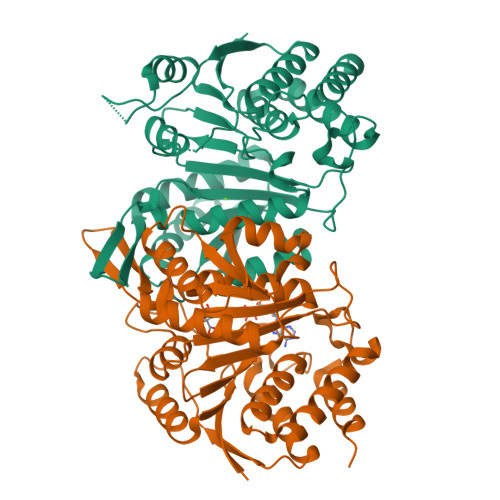> MGSTGGVQTVTLIPGDGIGPEISAAVMKIFDAAKAPIQWEERNVTAIQGPGGKWMIPSEAKESMDKNKMGLKGPLKTPIAAGHPSMNLLLRKTFDLYANVRPCVSIEGYKTPYTDVNIVTIRENTEGEYSGIEHVIVDGVVQSIKLITEGASKRIAEFAFEYARNNHRSNVTAVHKANIMRMSDGLFLQKCREVAESCKDIKFNEMYLDTVCLNMVQDPSQFDVLVMPNLYGDILSDLCAGLIGGLGVTPSGNIGANGVAIFESVHGTAPDIAGKDMANPTALLLSAVMMLRHMGLFDHAARIEAACFATIKDGKSLTKDLGGNAKCSDFTEEICRRVKDLD;> MGSFSEQTIPPSAKYGGRHTVTMIPGDGIGPELMLHVKSVFRHACVPVDFEEVHVSSNADEEDIRNAIMAIRRNRVALKGNIETNHNLPPSHKSRNNILRTSLDLYANVIHCKSLPGVVTRHKDIDILIVRENTEGEYSSLEHESVAGVVESLKIITKAKSLRIAEYAFKLAQESGRKKVTAVHKANIMKLGDGLFLQCCREVAARYPQITFENMIVDNTTMQLVSRPQQFDVMVMPNLYGNIVNNVCAGLVGGPGLVAGANYGHVYAVFETATRNTGKSIANKNIANPTATLLASCMMLDHLKLHSYATSIRKAVLASMDNENMHTPDIGGQGTTSEAIQDVIRHIRVINGRAVEA> GSSGSSGPVRFQEALKDLEVLEGGAATLRCVLSSVAAPVKWCYGNNVLRPGDKYSLRQEGAMLELVVRNLRPQDSGRYSCSFGDQTTSATLT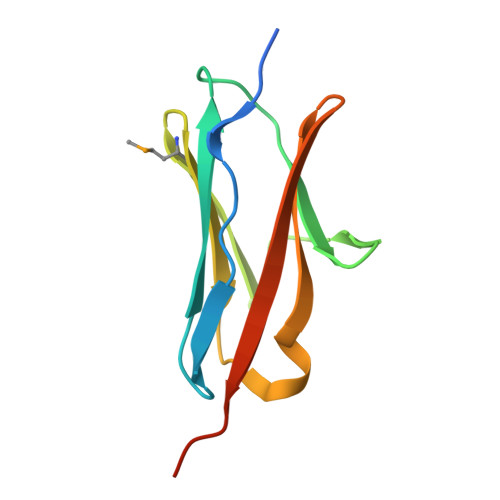VTALPSGPSSG> GSHMNGEPDIAQLKGLSPSQRQAYAVQLKNRGNHFFTAKNFNEAIKYYQYAIELDPNEPVFYSNISACYISTGDLEKVIEFTTKALEIKPDHSKALLRRASANESLGNFTDAMFDLSVLSLNGDFDGASIEPMLERNLNKQAMKVLNENLSKDEGRGSQVLPSNTSLASFFGIFDSHLEVSSVNTSSNYDTAYALLSDALQRLYSATDEGYLVANDLLTKSTDMYHSLLSANTVDDPLRENAALALCYTGIFHFLKNNLLDAQVLLQESINLHPTPNSYIFLALTLADKENSQEFFKFFQKAVDLNPEYPPTYYHRGQMYFILQDYKNAKEDFQKAQSLNPENVYPYIQLACLLYKQGKFT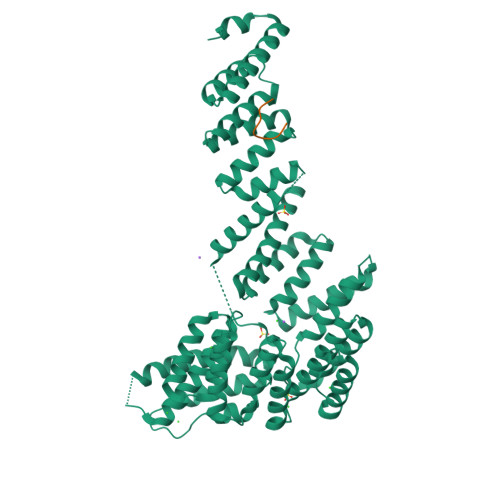ESEAFFNETKLKFPTLPEVPTFFAEILTDRGDFDTAIKQYDIAKRLEEVQEKIHVGIGPLIGKATILARQSSQDPTQLDEEKFNAAIKLLTKACELDPRSEQAKIGLAQLKLQMEKIDEAIELFEDSAILARTMDEKLQATTFAEAAKIQKRLRADPIISAKMELTLARYRAKGML;> GADNGPTVEEVD Talin rod domain–containing protein 1 (TLNRD1) shares 22% homology with the talin R7R8 rod domains, and is highly conserved throughout vertebrate evolution, although little is known about its function. Here we show that TLNRD1 is an α-helical protein structurally homologous to talin R7R8. Like talin R7R8, TLNRD1 binds F-actin, but because it forms a novel antiparallel dimer, it also bundles F-actin. Increasing TLNRD1 expression enhances filopodia formation and cell migration on 2D substrates, while TLNRD1 down-regulation has the opposite effect. Together, our results suggest that TLNRD1 has retained the diverse interactions of talin R7R8, but has developed distinct functionality as an actin-bundling protein that promotes filopodia assembly.

To determine the extent of the structural similarity between TLNRD1 and talin R7R8, we used x-ray crystallography to solve the structures of both full-length TLNRD1 (TLNRD1-FL) and the four-helix domain (TLNRD1-4H). In both the TLNRD1-FL and TLNRD1-4H structures, the four-helix bundle forms an extensive interaction with a four-helix bundle of a second TLNRD1 molecule. An identical dimer interface was observed in both the TLNRD1-FL and the TLNRD1-4H structures, which crystallized in different space groups. Dimerization of TLNRD1 is mediated via an extensive hydrophobic interface on helices α6 and α7, with the two F250 side chains docking into the opposing molecule. The surface of each four-helix bundle has a pocket created by F270’ and the small side chains of G217’ and A260’ that the F250 aromatic rings docks into. As it is a symmetric dimer, the F250’ docks into the equivalent pocket on the other molecule, leading to an antiparallel configuration. The interface is capped at either end by electrostatic interactions between the side chains of E267 and R246’ and vice versa. TLNRD1-4H bound to RIAM with similar affinity (Kd 0.59 µM), confirming the RIAM interaction is mediated by the four-helix domain. Last, no interaction was observed between KANK1 and TLNRD1-4H, confirming the TLNRD1-KANK1 interaction is mediated via the five-helix module. Given the discovery that TLNRD1-4H can bind actin filaments, we tested the ability of TLNRD1-4H to bundle actin, and surprisingly, we found that the four-helix domain alone is an effective actin bundler.

> GGSAQPGLVDRYRVTRCRHEVEQGCAVLRATPLADMTPQLLLEVSQGLSRNLKFLTDACALASDKSRDRFSREQFKLGVKCMSTSASALLACVREVKVAPSELARSRCALFSGPLVQAVSALVGFATEPQFLGR> QNLDSMLHGTGMKSDSDQKKSENGVTLAPEDTLPFLKCYCSGHCPDDAINNTCITNGHCFAIIEEDDQGETTLASGCMKY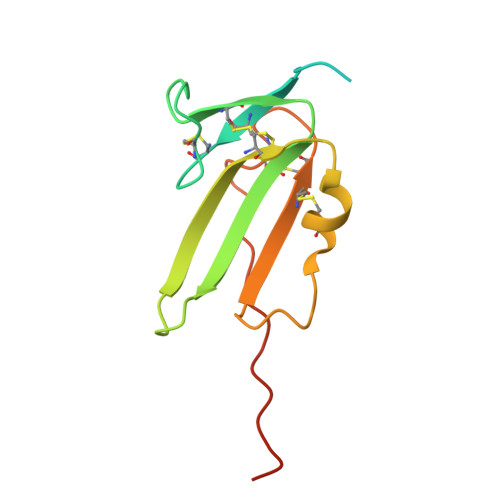EGSDFQCKDSPKAQLRRTIECCRTNLCNQYLQPTLPPVVIGPFFDGSIR IMINORIBITOL | C5 H11 N O3 | 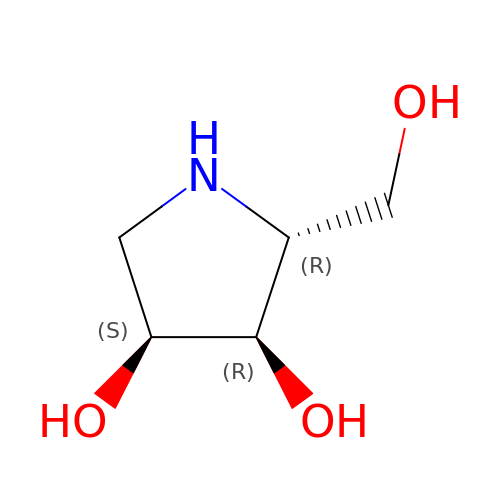OQEBIHBLFRADNM-MROZADKFSA-N> ESQPDPTPDELHKSSEFTGTMGNMKYLYDDHYVSATKVMSVDKFLAHDLIYNISDKKLKNYDKVKTELLNEDLAKKYKDEVVDVYGSNYYVNCYFSSKDNVGKVTGGKTCMYG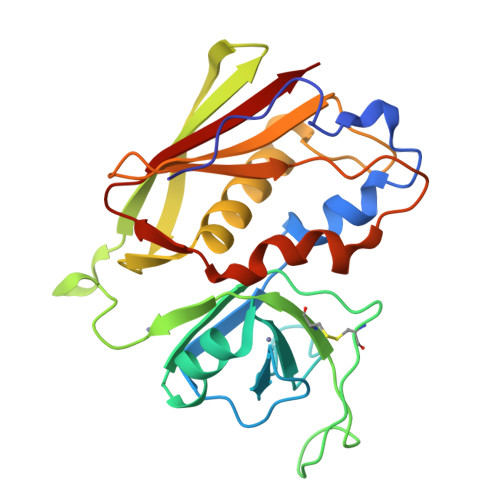GITKHEGNHFDNGNLQNVLIRVYENKRNTISFEVQTDKKSVTAQELDIKARNFLINKKNLYEFNSSPYETGYIKFIENNGNTFWYDMMPAPGDKFDQSKYLMMYNDNKTVDSKSVKIEVHLTTKNG> M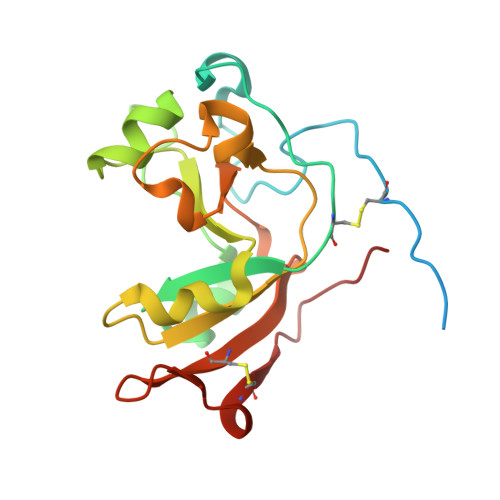GSSHHHHHHSSGENLYFQGSHMTATATSAKAAAPACPRFDDPVHAAADPRVDVERITPDPVWRTTCGTLYRSDSRGPAVVFEQGFLPKDVIDGQYDIESYVLVNQPSPYVATTYDHDLYKTWYKSGYNYYIDAPGGVDVNKTIGDRHKWADQVEVAFPGGIRTEFVIGVCPVDKKTRTEKMSECVGNPHYEPWH>MALSTATKAATDALAANRAPTSVNAQEVHRWLQSFNWDFKNNRTKYATKYKMANETKEQFKLIAKEYARMEAVKDERQFGSLQDALTRLNAGVRVHPKWNETMKVVSNFLEVGEYNAIAATGMLWDSAQAAEQKNGYLAQVLDEIRHTHQCAYVNYYFAKNGQDPAGHNDARRTRTIGPLWKGMKRVFSDGFISGDAVECSLNLQLVGEACFTNPLIVAVTEWAAANGDEITPTVFLSIETDELRHMANGYQTVVSIANDPASAKYLNTDLNNAFWTQQKYFTPVLGMLFEYGSKFKVEPWVKTWDRWVYEDWGGIWIGRLGKYGVESPRSLKDAKQDAYWAHHDLYLLAYALWPTGFFRLALPDQEEMEWFEANYPGWYDHYGKIYEEWRARGCEDPSSGFIPLMWFIENNHPIYIDRVSQVPFCPSLAKGASTLRVHEYNGEMHTFSDQWGERMWLAEPERYECQNIFEQYEGRELSEVIAELHGLRSDGKTLIAQPHVRGDKLWTLDDIKRLNCVFKNPVKAFN[2x];>[2x]MSMLGERRRGLTDPEMAAVILKALPEAPLDGNNKMGYFVTPRWKRLTEYEALTVYAQPNADWIAGGLDWGDWTQKFHGGRPSWGNETTELRTVDWFKHRDPLRRWHAPYVKDKAEEWRYTDRFLQGYSADGQIRAMNPTWRDEFINRYWGAFLFNEYGLFNAHSQGAREALSDVTRVSLAFWGFDKIDIAQMIQLERGFLAKIVPGFDESTAVPKAEWTNGEVYKSARLAVEGLWQEVFDWNESAFSVHAVYDALFGQFVRREFFQRLAPRFGDNLTPFFINQAQTYFQIAKQGVQDLYYNCLGDDPEFSDYNRTVMRNWTGKWLEPTIAALRDFMGLFAKLPAGTTDKEEITASLYRVVDDWIEDYASRIDFKADRDQIVKAVLAGLK;>MAKLGIHSNDTRDAWVNKIAQLNTLEKAAEMLKQFRMDHTTPFRNSYELDNDYLWIEAKLEEKVAVLKARAFNEVDFRHKTAFGEDAKSVLDGTVAKMNAAKDKWEAEKIHIGFRQ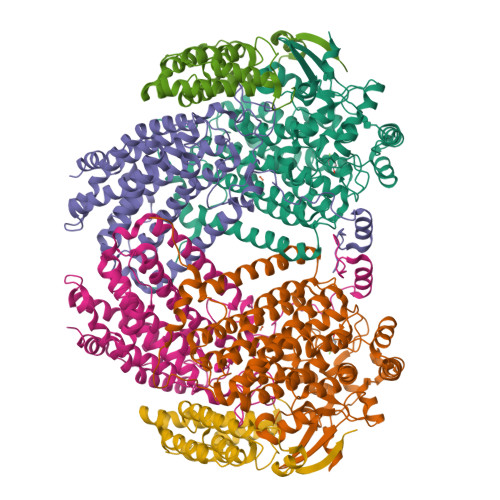AYKPPIMPVNYFLDGERQLGTRLMELRNLNYYDTPLEELRKQRGVRVVHLQSPH[2x]>GSGRVSLNFKDPEAVRALTCTLLREDFGLSIDIPLERLIPTVPLRLNYIHWVEDLIGHQDSDKSTLRRGIDIGTGASCIYPLLGATLNGWYFLAT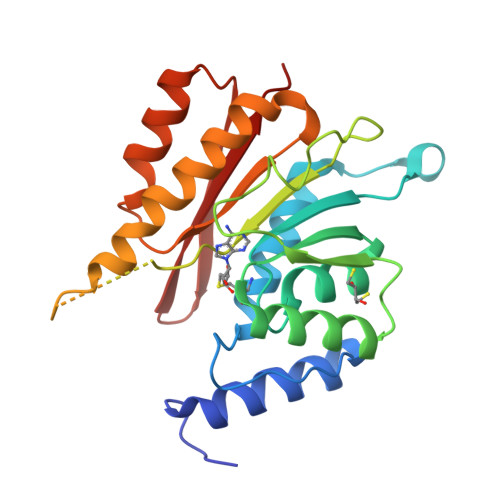EVDDMCFNYAKKNVEQNNLSDLIKVVKVPQKTLLMDALKEESEIIYDFCMCNPPFFANQLEAKGVNSRNPRRPPPSSVNTGGITEIMAEGGELEFVKRIIHDSLQLKKRLRWYSCMLGKKCSLAPLKEELRIQGVPKVTYTEFCQGRTMRWALAWSFYD[3x]> GPHMKYKLADYRYGREEMLA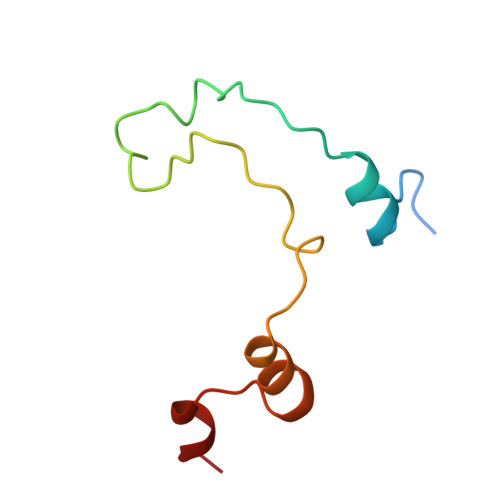LYVKENKVPEELQDKEFAAVLQDEPLQPLALEPLTEEEQRNFSLSVNSVAVLRLM> SPTVEECGYSDRVRSITLGNSTITTQECANVVVGYGEWPEYLSDNEATAEDQPTQPDVATCRFYTLDSVQWENGSPGWWWKFPDALRDMGLFGQNMYYHYLGRAGYTIHVQCNASKFHQGCILVVCVPEAEMGSAQTSGVVNYEHISKGEIASRFTTTTTAEDHGVQAAVWNAGMGV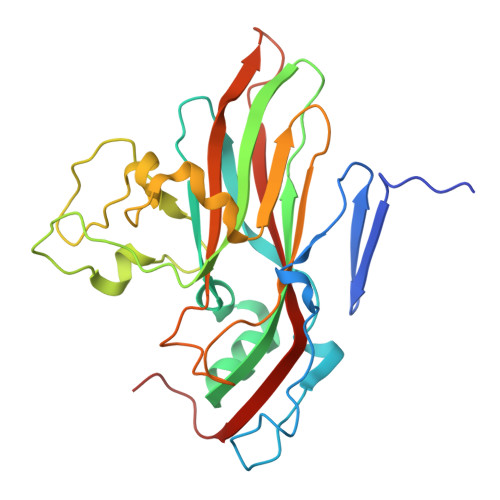GVGNLTIFPHQWINLRTNNSATIVMPYVNSVPMDNMYRHHNFTLMIIPFVPLDFSAGASTYVPITVTVAPMCAEYNGLRLAGHQ N~2~-[(2R)-2-(3,5-dichlorophenyl)-2-(dimethylamino)acetyl]-N-({2-[(Z)-iminomethyl]pyrimidin-4-yl}methyl)-L-isoleucinamide 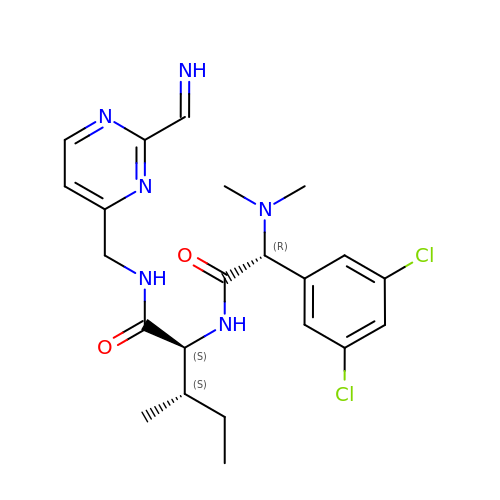| C22 H28 Cl2 N6 O2 | XBUAFLLXSYLZPV-GKZFGAONSA-N>[4x]SFRDCAEVFKSGHTTNGIYTLTFPNSTEEIKAYCDMEAGGGGWTIIQRREDGSVDFQRTWKEYKVG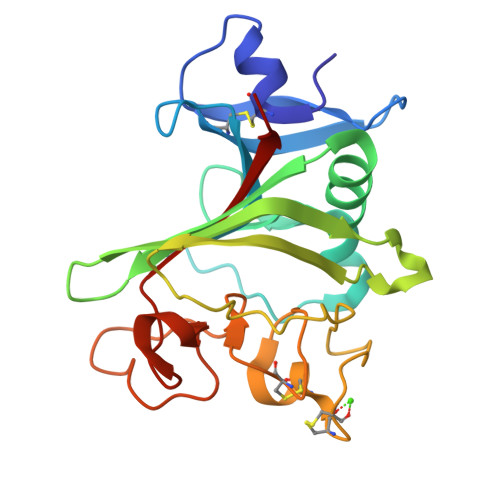FGNPSGEYWLGNEFVSQLTNQQRYVLKIHLKDWEGNEAYSLYEHFYLSSEELNYRIHLKGLTGTAGKISSISQPGNDFSTKDGDNDKCICKCSQMLTGGWWFDACGPSNLNGMYYPQRQNTNKANGIKWAAWKGSGYSLKATTMMIRPADF> GDSIEDKNARVIELIAAYRNRGHLMADIDPLRLDNTRFRSHPDLDVNSHGLTLWDLDREFKVDGFAGVQRKKLRDILSVLRDAYCRHVGVEYTHILEPEQQRWIQERVETKHDKPTVAEQKYILSKLNAAEAFETFLQTKYVGQKRFSLEGAETVIPMMDAVIDQCAEH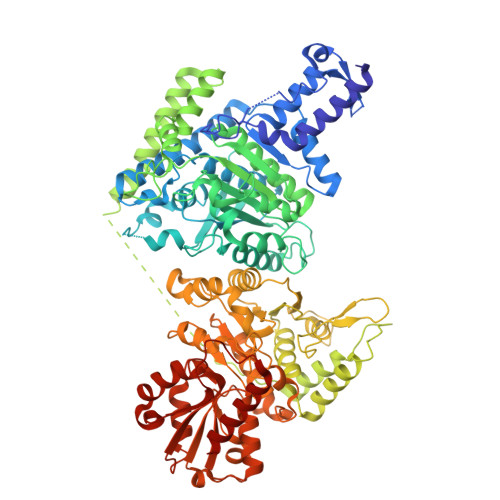GLDEVVIAMPHRGRLNVLANIVGKPYSQIFSEFEGNLNPSQAHGSGDVKYHLGATGTYIQMFGDNDIEVSLTANPSHLEAVDPVLEGLVRAKQDLLDTGEEGSDNRFSVVPLMLHGDAAFAGQGVVAETLNLALLRGYRTGGTIHIVVNNQIGFTTAPTDSRSSEYCTDVAKMIGAPIFHVNGDDPEACAWVARLAVDFRQAFKKDVVIDMLCYRRRGHNEGDDPSMTQPYMYDVIDTKRGSRKAYTEALIGRGDISMKEAEDALRDYQGQLEAVFNEVRELEKHEIEPSESVEADQQIPSKLATAVDKAMLQRIGDAHLALPEGFTVHPRVRPVLEKRREMAYEGRIDWAFAELLALGSLIAEGKLVRLSGQDTQRGTFTQRHAVIVDRKTGEEFTPLQLLATNPDGTPTGGKFLVYNSALSEFAAVGFEYGYSVGNPDAMVLWEAQFGDFVNGAQSIIDEFISSGEAKWGQLSDVVLLLPHGHEGQGPDHTSGRIERFLQLWAEGSMTIAMPSTPANYFHLLRRHGKDGIQRPLIVFTPKSMLRNKAAVSDIRDFTESKFRSVLEEPMYTDGEGDRNKVTRLLLTSGKIYYELAARKAKENREDVAIVRIEQLAPLPRRRLAETLDRYPNVKEKFWVQEEPANQGAWPSFGLTLPEILPDHFTGLKRISRRAMSAPSSGSSKVHAVEQQEILDTAFG>[2x]MGDNIVLYYFDARGKAELIRLIFAYLGIEYTD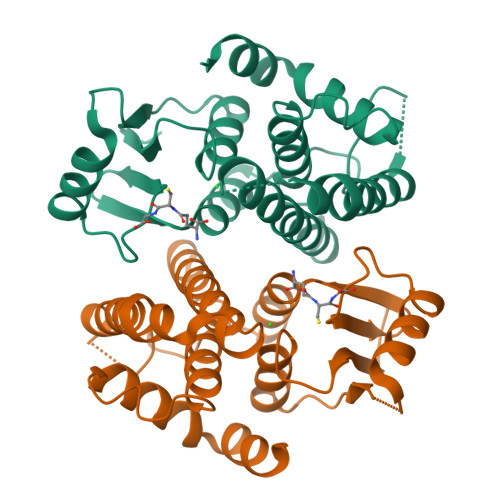KRFGVNGDAFVEFKNFKKEKDTPFEQVPILQIGDLILAQSQAIVRYLSKKYNICGESELNEFYADMIFCGVQDIHYKFNNTNLFKQNETTFLNEDLPKWSGYFEKLLKKNHTNNNNDKYYFVGNNLTYADLAVFNLYDDIETKYPSSLKNFPLLKAHNEFISNLPNIKNYITNRKESVY A prominent member of these so-called Knallgas bacteria is Cupriavidus necator H16 (formerly Ralstonia eutropha H16), which employs four different O2-tolerant [NiFe]-hydrogenases for generating cellular energy from the controlled oxidation of H2 in the presence of O2.5 Among them, only the tripartite membrane-bound [NiFe]-hydrogenase (MBH) is directly linked to the respiratory chain. The MBH large subunit contains the catalytic center composed of a nickel and an iron ion, which are coordinated to the protein by four Cys-derived thiolates. The most distal cluster relative to the active site is a [4Fe–4S] cluster coordinated by three cysteines and a histidine, while the medial cluster is a [3Fe–4S] species with three cysteines as protein anchors. However, in the proximal position, instead of a standard Cys4[4Fe–4S] cluster, the O2-tolerant MBHs possess a [4Fe–3S] cluster coordinated by six cysteine residues (Fig. 1 and S1†).13–16 The unique architecture of the [4Fe–3S] cluster is associated with a redox-dependent structural flexibility that allows two redox-transitions within a physiological potential region, i.e., the cofactor can assume a super-oxidized, an oxidized, and a reduced state. In order to obtain insight into the individual role of the supernumerary cysteines in the coordination and function of the [4Fe–3S] cluster, we purified C. necator MBH derivatives carrying exchanges of cysteine for glycine at the positions 19 and/or 120 in the small subunit HoxK, which are hereafter referred to as MBHC19G, MBHC120G and MBHC19G/C120G.

Even in the MBHC19G/C120G protein, which contains a four Cys-coordinated [4Fe–4S] species, oxidation resulted in cluster flexibility, indicating that the binding pocket is optimized for an Fe–S cluster of larger dimensions, i.e., the Cys6[4Fe–3S] cluster. The function of the Cys19-derived thiolate bridging Fe1 and Fe4 in the native [4Fe–3S] cluster, was taken over by the additional sulfide S4, which also formed a covalent bond to Fe3. Oxidized crystals of the same variant diffracted with a resolution of up to 1.65 Å (Table S2†). The corresponding crystal structure also showed a “cubane-like” [4Fe–4S] cluster with some structural flexibility of the Fe3, S1 and S3 positions compared to the reduced MBHC19G/C120G. Interestingly, the mFo-DFc electron density maps of both oxidized and reduced MBHC19G/C120G uncovered a positive density at the former position of Cys120, which is most likely a water molecule based on SAD data (Fig. 2d and S4d†). Thus, the Cys4[4Fe–4S] cluster in MBHC19G/C120G is similar but not identical to the classical Cys4[4Fe–4S] cluster of O2-sensitive [NiFe]-hydrogenases. In addition to MBHC19G and MBHC120G, the oxidized MBHC19G/C120G protein forms preferentially the Nir-B state, showing that the manifold engineered proximal clusters does not necessarily lead to accumulation of Niu-A.

> MSAYATQGFNLDDRGRRIVVDPVTRIEGHMRCEVNVDANNVIRNAVSTGTMWRGLEVILKGRDPRDAWAFVERICGVCTGCHALASVRAVENALDIRIPKNAHLIREIMAKTLQVHDHAVHFYHLHALDWVDVMSALKADPKRTSELQQLVSPAHPLSSAGYFRDIQNRLKRFVESGQLGPFMNGYWGSKAYVLPPEANLMAVTHYLEALDLQKEWVKIHTIFGGKNPHPNYLVGGVPCAINLDGIGAASAPVNMERLSFVKARIDEIIEFNKNVYVPDVLAIGTLYKQAGWLYGGGLAATNVLDYGEYPNVAYNKSTDQLPGGAILNGNWDEVFPVDPRDSQQVQEFVSHSWYKYADESVGLHPWDGVTEPNYVLGANTKGTRTRIEQIDESAKYSWIKSPRWRGHAMEVGPLSRYILAYAHARSGNKYAERPKEQLEYSAQMINSAIPKALGLPETQYTLKQLLPSTIGRTLARALESQYCGEMMHSDWHDLVANIRAGDTATANVDKWDPATWPLQAKGVGTVAAPRGALGHWIRIKDGRIENYQCVVPTTWNGSPRDYKGQIGAFEASLMNTPMVNPEQPVEILRTLHSFDPCLACSTH;> METKPRTPVLWLHGLECTGCSESFIRSAHPLAKDVVLSMISLDYDDTLMAAAGHQAEAILEEIMTKYKGNYILAVEGNPPLNQDGMSCIIGGRPFIEQLKYVAKDAKAIISWGSCASWGGVQAAKPNPTQATPVHKVITDKPIIKVPGCPPIAEVMTGVITYMLTFDRIPELDRQGRPKMFYSQRIHDKCYRRPHFDAGQFVEEWDDESARKGFCLYKMGCKGPTTYNACSTTRWNEGTSFPIQSGHGCIGCSEDGFWDKGSFYDRLTGISQFGVEANADKIGGTASVVVGAAVTAHAAASAIKRASKKNETSGSEHRSAWSHPQFEK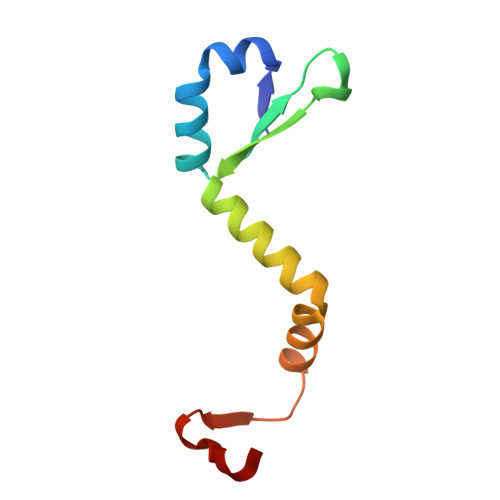> MIITSPTEARKDFYQLLKNVNNNHEPIYISGNNAENNAVIIGLEDWKSIQETIYLESTGTMDKVREREKDNSGTTNIDDIDWDNL>[3x]MMSIAQVRSAGSAGNYYTDKDNYYVLGSMGERWAGRGAEQLGLQGSVDKDVFTRLLEGRLPDGADLSRMQDGSNRHRPGYDLTFSAPKSVSMMAMLGGDKRLIDAHNQAVDFAVRQVEALASTRVMTDGQSETVLTGNLVMALFNHDTSRDQEPQLHTHAVVANVTQHNGEWKTLSSDKVGKTGFIENVYANQIAF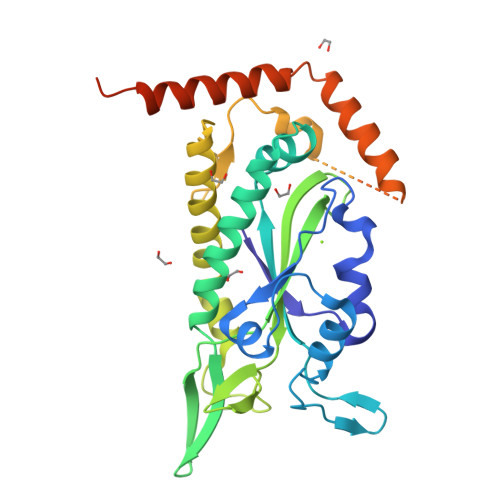GRLYREKLKEQVEALGYETEVVGKHGMWEMPGVPVEAFSGRSQTIREAVGEDASLKSRDVAALDTRKSKQHVDPEIKMAEWMQTLKETGFDIRAYRDAADQRADLRTLTPGPASQDGPDVQQAVTQAIAGLSER> SMFEFDNLAPMLATHGTVAGLKASQWAFEGMWDGYRLLVEADHGAVRLRSRSGRDVTAEYPQLRALAEDLADHHVVLDGEAVVLDSSGVPSFSQMQNRGRDTRVEFWAFDLLYLDGRALLGTRYQDRRKLLETLANATSLTVPELLPGDGAQAFACSRKHGWEGVIAKRRDSRYQPGRRCASWVKDKHWNTQEVVIGGWRAGEGRSGVGSLLMGIPGPGGLQFAGRVGTGLSERELANLKEMLAPLHTDESPFDVPLPARDAKGITYVKPALVAEVRYSEWTPEGRLRQSSW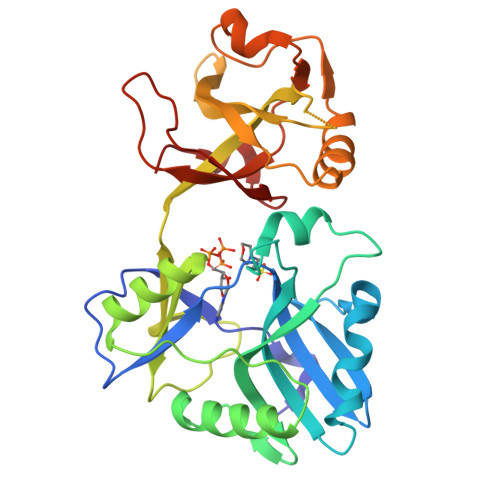RGLRPDKKPSEVVRE> KLSEHLRYCDSILREMLSKKHAAYAWPFYKPVDAEALELHDYHDIIKHPMDLS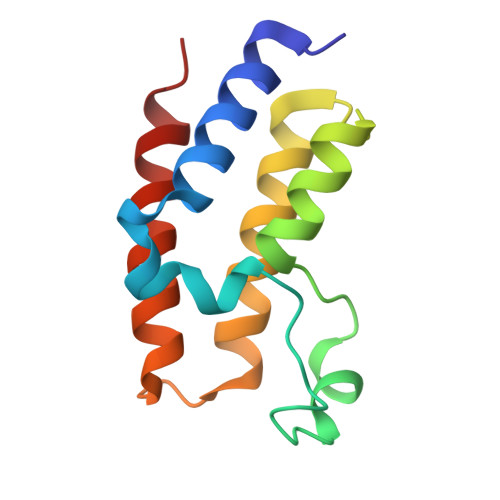TVKRKMDGREYPDAQGFAADVRLMFSNCYKYNPPDHEVVAMARKLQDVFEMRFAKMP> LKCNQLIPPFWKTCPKGKNLCYKMTMRAA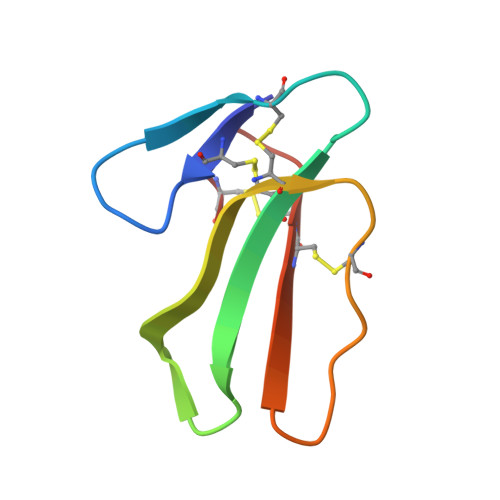PMVPVKRGCIDVCPKSSLLIKYMCCNTDKCN>MDSIQAEEWYFGKITRRESERLLLNAENPRGTFLVRESETTKGAYSLSVSDFDNAKGLNVKHYKIRKLDSGGFYI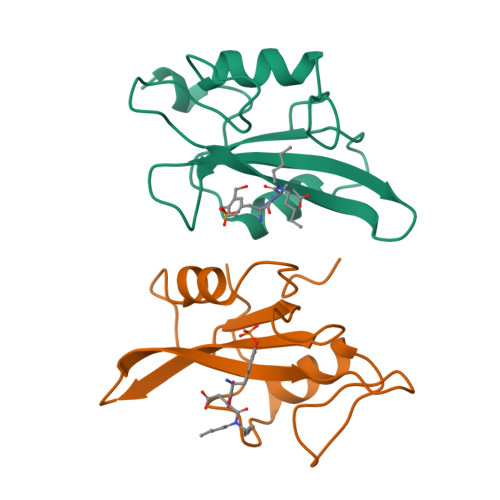TSRTQFNSLQQLVAYYSKHADGLCHRLTTVCP[2x]>MPMILGYWDIRGLAHAIRLLLEYTDSSYEEKKYTMGDAPDYDRSQWLNEKFKLGLDFPNLPYLIDGAHKITQSNAILCYIARKHNLCGETEEEKIRVDILENQTMDNHMQLGMICYNPEFEKLKPKYLEELPEKLKLYSEFLGKRPWFAGNKITFVDFLVYDVLDLHRIFEPKCLDAFPNLKDFISRFEGLEKISAYMKSSRFLPRPVFSKMAVWG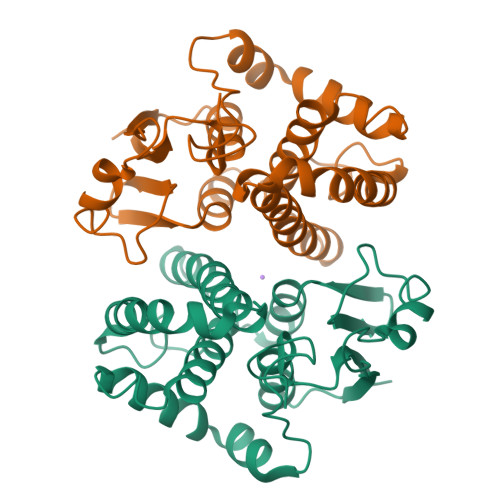NK[4x]>[5x]GSHM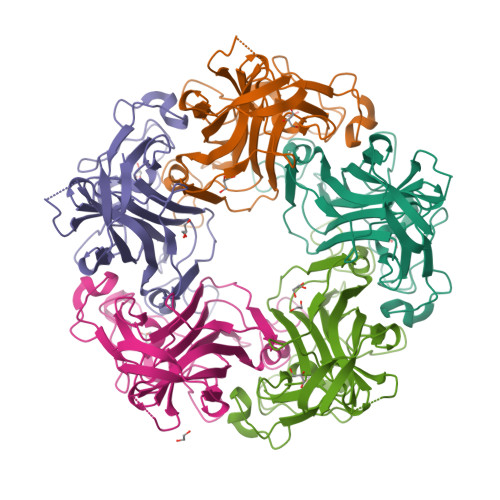GGVEVLEVKTGVDSITEVECFLTPEMGDPDEHFRGFSKSISISDTFESDSPNRDMLPCYSVARIPLPNLNEDLTCGNILMWEAVTLKTEVIGVTSLMNVHSNGQATHDNGAGKPVQGTSFHFFSVGGEALELQGVLFNYRTKYPDGTIFPKNATVQSQVMNTEHKAYLDKNKAYPVECWVPDPTRNENTRYFGTLTGGENVPPVLHITNTATTVLLDEFGVGPLCKGDNLYLSAVDVCGMFTNRSGSQQWRGLSRYFKVQLRKRRVKN>ASGADALKALNKDNDDSLEIAEVIHAGATTFTAINPDGDTTLESGETKGRLTEKDWARANKDGDQTLEMDEWLKILRTRFKRADANKDGKL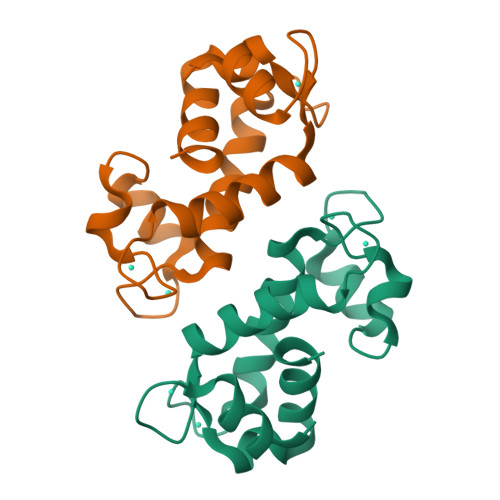TAAELDSKAGQGVLVMIMK[4x]>EDPHLRNRPGKGHNYIDGMTQEDATCKPVTYAGACSSFDVLLEKGKFPLFQSYAHHRTLLEAVHDTIIAKADPPSCDLQSAHGNPCMKEKLVMKTHCPNDYQSAHYLNNDGKMASVKCPPKYELTEDCNFCRQMTGASLKKGSYPLQDLFCQSSEDDGSKLKTKMKGVCEVGVQALKKCDGQLSTAHEVVPFAVFKNSKKVYLDKLDLKTEENLLPDSFVCFEHKGQYKGKLDSGQTKRELKSFDISQCPKIGGHGSKKCTGDAAFCSAYECTAQYANAYCSHANGSGIVQIQVSGVWKKPLCVGYERVVVKRELS[5x];>DPGCSELIQASSRITTCSTEGVNTKCRLSGTALIRAGSVGAEACLMLKGVKEDQTKFLKIKTVSSELSCREGQSYWTGSFSPKCLSSRRCHLVGECHVNRCLSWRDNETSAEFSFVGESTTMRENKCFEQCGGWGCGCFNVNPSCLFVHTYLQSVRKEALRVFNCIDWVHKLTLEITDFDGSVSTIDLGASSSRFTNWGSVSLSLDAEGISGSNSFSFIESPGKGYAIVDEPFSEIPRQGFLGEIRCNSESSVLSAHESCLRAPNLISYKPMIDQLECTTNLIDPFVVFERGSLPQTRNDKTFAASKGNRGVQAFSKGSVQADLTLMFDNFEVDFVGAAVSCDAAFLNLTGCYSCNAGARVCLSITSTGTGSLSAHNKDGSLHIVLPSENGTKDQCQILHFTVPEVEEEFMYSCDGDERPLLVKGTLIAID[5x]

Rift Valley fever virus (RVFV; genus phlebovirus, family Phenuiviridae) is an important example of an enveloped virus that harbours a class II fusion protein. As with other phleboviruses, RVFV displays two glycoproteins on the lipid bilayer envelope of the virion, Gn and Gc, which form higher order pentameric and hexameric ring-shaped assemblies. While the Gc glycoprotein is responsible for membrane fusion, the role of the Gn remains undefined. Virus entry is completed upon Gc-mediated fusion of the viral envelope and host cell membrane, in a pH-dependent mechanism.

Localized reconstruction of each of the four types of the Gn–Gc capsomers (pentamers and hexamers of type 1–3) resulted in four independent structures at resolutions between 7.7 and 8.6-Å. We first performed fitting with the localized reconstruction of the pentamer at 7.7 Å resolution, followed by fitting the resulting Gn–Gc heterodimer model to localized reconstructions of the hexamers at 8.0–8.6 Å resolution. Consistent with previous biochemical and structural studies, this fitting verified that the Gn and Gc assemble as heterodimers, which form higher order ring-like pentameric and hexameric capsomer structures on the mature virion. Domain A of the Gn forms a ring on top of these capsomers interacting with domain II of Gc, occluding a surface area of ~950 Å2. The Gn–Gc interface is formed between the β-ribbon domain of the Gn and the hydrophobic fusion loops of Gc11, which are shielded from solvent at the interface between Gn domains A and B. Surprisingly, unlike the rod-like array of extended anti-parallel Gc dimers predicted from the low-resolution modelling attempts, we observed that RVFV Gc forms a kinked conformation, not previously sampled in crystallographic investigations of class II fusion glycoproteins. Sub-tomogram averaging and MDFF fitting revealed that while non-membrane-facing capsomers retain the pre-fusion configuration, membrane-interacting pentamers undergo pronounced conformational rearrangements that allow the insertion of the Gc-residue hydrophobic fusion loops into the target membrane. This insertion event is achieved, in part, by a dramatic translational shift of the Gn, which unshields the Gc allowing it to form an extended intermediate state. Although it is tempting to speculate that the pentamers might have a lower activation barried to escape their metastable state than the hexamers, possibly due to less favourable subunit–subunit angles (72° in the 60 heterodimers making the pentamers as opposed to ~60° in the 660 heterodimers making the hexamers), this hypothesis remains to be tested.Clathrin mediates vesicular transport between post‐Golgi membranes in eukaryotes and is targeted to specific membranes by interactions with clathrin adaptor proteins. A total of 3 consensus clathrin‐binding peptide sequences have been identified and structural studies show that each binds distinct sites on the clathrin heavy chain N‐terminal domain (NTD). We have solved high‐resolution structures of NTD bound to peptide motifs from the cellular clathrin adaptors β2 adaptin and amphiphysin plus a putative viral clathrin adaptor, hepatitis D virus large antigen (HDAg‐L). Surprisingly, with each peptide we observe simultaneous peptide binding at multiple sites on NTD and viral peptides binding to the same sites as cellular peptides.

In all the structures presented a peptide could be observed at the “clathrin box”, lying between blades 1 and 2 of the NTD β‐propeller fold (“clathrin box”). For the cellular peptides (AP2CBMpep, AmphCBMpep and Amph4T1pep) the binding is similar to that previously described, with the 3 leucine side chains of the CBM LΦxΦ[DE] consensus sequence occupying the hydrophobic pocket formed at the groove between the 2 blades. In addition to binding at the clathrin box, we observed significant binding of the cellular peptides (AP2CBMpep, AmphCBMpep and Amph4T1pep) at the “arrestin box”, which lies between blades 4 and 5 of the NTD β‐propeller fold (“arrestin box”). While all 3 CBM peptides bind in the same general orientation at the arrestin box, the molecular details of these interactions differ from the interaction seen between NTD and the extended surface loop of the arrestin 2 long isoform (arrestin2L). Most notably, the directionality of the peptide chain is reversed. The first 2 leucine residues of each CBM (LΦxΦ[DE]) bind in a hydrophobic cavity lined by the side chains of NTD residues W164, L183, S185, R188, V190, I194, F216, I231 and V233 plus the peptide backbones of Y184 and S191. In the structures presented here the side chain oxygen atom of NTD residue Q192 forms hydrogen bonds with the backbone amide protons of these 2 leucine residues (LΦxΦ[DE]) and the side chain nitrogen atom of Q192 forms a hydrogen bond with the carbonyl oxygen of the second leucine (LΦxΦ[DE]). In the AmphCBMpep structure the side chain of the phenylalanine residue that follows the CBM forms an additional hydrophobic interaction with NTD, binding in a hydrophobic cleft formed by side chains of residues H229, I231 and A247, the aryl side chain region of K245, and the peptide backbones of residues 245‐247. However, unlike at the arrestin box, residues that form the molecular interactions at the Royle box do not correspond to those conserved in the LΦxΦ[DE] consensus CBM sequence and we note that several peptides containing a CBM sequence (AP2CBMpep, AmphCBMpep and AmphCBMlongpep) do not bind at the Royle box.

>[2x]GSMAQILPIRFQEHLQLQNLGINPANIGFSTLTMESDKFICIREKVGEQAQVVIIDMNDPSNPIRRPISADSAIMNPASKVIALKAGKTLQIFNIEMKSKMKAHTMTDDVTFWKWISLNTVALVTDNAVYHWSMEGESQPVKMFDRHSSLAGCQIINYRTDAKQKWLLLTGISAQQNRVVGAMQLYSVDRKVSQPIEGHAASFAQFKMEGNAEESTLFCFAVRGQAGGKLHIIEVGTPPTGNQPFPKKAVDVFFPPEAQNDFPVAMQISEKHDVVFLITKYGYIHLYDLETGTCIYMNRISGETIFVTAPHEATAGIIGVNRKGQVLSVCVEEENIIPYITNVLQNPDLALRMAVRNNLAGAEEL;>[4x]ETLLDLDFDP>[2x]MGSHHHHHHSQDPMMSRLKTAVYDYLNDVDITECTEMDLLCQLSNCCDFINETYAKNYDTLY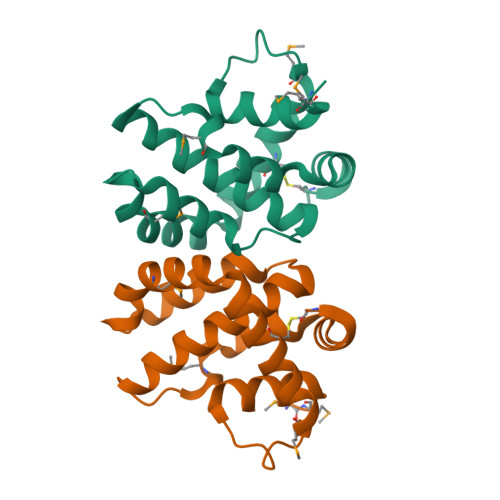DIMERDILSYNIVNIKNTLTFALRDASPSVKLATLTLLASVIKKLNKIQHTDAAMFSEVIDGIVAEEQQVIGFIQKKCKYNTT> SFEDKPWRKPGA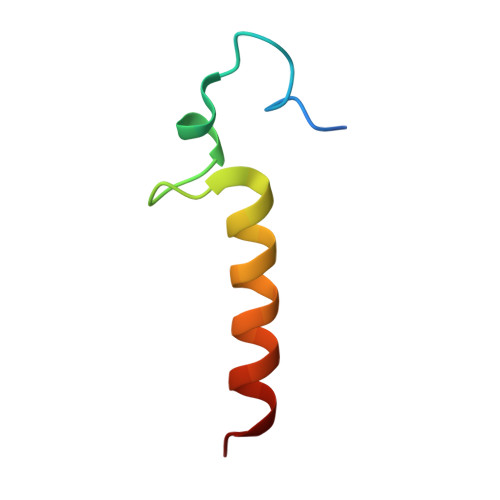DLSDYFNYGFNEDTWKAYCEKQKRIRMGLE> AKRHRKVLR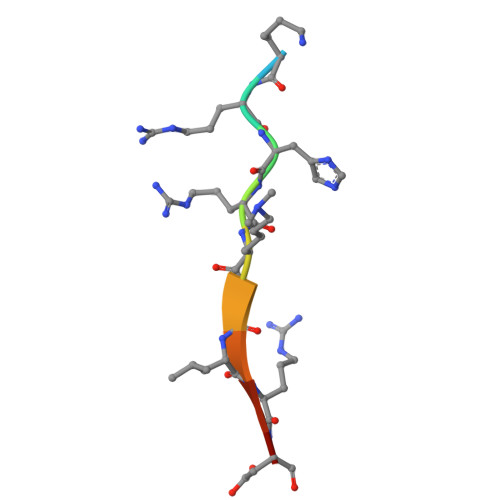DN Most cyanobacterial strains produce extracellular polymeric substances (EPS), mainly composed of heteropolysaccharides that can remain attached to the cell surface (CPS—capsular polysaccharides) or be released into the environment (RPS—released polysaccharides). Wzc undergoes a phospholyation/dephosphorylation cycle that affects its oligomerization state and is dependent on the phosphatase activity of another protein, Wzb (Cuthbertson, Mainprize, Naismith, & Whitfield, 2009). In addition, Sll0328 was identified as a low molecular weight protein tyrosine phosphatase (LMW‐PTP; EC: 3.1.3.48) and Wzb homolog. Most importantly, Wzb was able to dephosphorylate Wzc in vitro, suggesting that tyrosine phosphorylation/dephosphorylation plays a role in cyanobacterial EPS production.

The structure of Wzb was solved (2.28 Å), revealing structural differences relative to other phosphatases involved in EPS production and suggesting a different substrate recognition mechanism. One monomer was present in the asymmetric unit, with the crystal lattice belonging to the P312 1 space group. Synechocystis’ Wzb displays the structure of a low molecular weight protein tyrosine phosphatase (LMW‐PTP). The PTPases signature motif, the PTP loop, with the characteristic sequence C(X)5R(S/T) (cysteine 7 to serine 14) is located between the C‐terminus of the β1 strand and the N‐terminus of the α1 helix, at the N‐terminus side of the protein. Opposite and topping this loop, there is the DPYY loop, which contains the functionally essential aspartate residue (D124). Together, the DPYY and PTP loops constitute the enzyme´s active site. The tyrosine residues of the DPYY loop form one of the walls of the active site pocket, with a histidine (H45) delineating the other side of the substrate entry site. Two features of the Wzb structure are particularly relevant for its functional properties: (a) it possesses the second Y of the DPYY motif (Y127) that is absent in most prokaryotic LMW‐PTPs (Bohmer, Szedlacsek, Tabernero, Ostman, & Hertog, 2013; Lescop et al., 2006; Standish & Morona, 2014). (b) Synechocystis’ Wzb possesses an aromatic residue—histidine (H45)—in the catalytic site instead of the hydrophobic leucine that occupies this position in most prokaryotic LMW‐PTPs. Based on these characteristics, Synechocystis Wzb can be classified as a class I or eukaryotic‐like LMW‐PTP and is therefore likely to present a substrate recognition mechanism different from that of E. coli Wzb, a class II or prokaryotic‐like LMW‐PTPs.

> MRGSHHHHHHGSACKLLFVCLGNICRSPAAENIMNAQIDQAGLGAKIVCDSAGTSSYHVGDSPDRRMTESLKKRGYRVQGRARQFFPEDFAEFDLILAMDGDNYRNILAQDPAGQYHHKVKMICDYTEKFGDREVPDPYYGGQAGFEHVIDLLEDACGNLLTSLGKELVN>GFKDNSPISDTSFSLQLSQDGLQLTPASSSSESLSIIDVASDQNLFQTFIKEWRCKKRFSISLACEKIRSLTSSKTATIGSRFKQASSPQEIPIRDDGFPIKGCDDTLVVGLAVCWGGRDAYYFSLQKEQKHSEISASLVPPSLDPSLTLKDRMWYLQSCLRKESDKECSVVIYDFIQSYKILLLSCGISLEQSYEDPKVACWLLDPDSQEPTLHSIVTSFLPHELPLLEGMETSQGIQSLGLNAGSEHSGRYRASVESILIFNSMNQLNSLLQKENLQDVFRKVEMPSQYCLALLELNGIGFSTAECESQKHIMQAKLDAIETQAYQLAGHSFSFTSSDDIAEVLFLELKLPPNREMKNQGSKKTLGSTRRGIDNGRKLRLGRQFSTSKDVLNKLKALHPLPGLILEWRRITNAITKVVFPLQREKCLNPFLGMERIYPVSQSHTATGRITFTEPNIQNVPRDFEIKMPTLVGESPPSQAVGKGLLPMGRGKYKKGFSVNPRCQAQMEERAADRGMPFSISMRHAFVPFPGGSILAADYSQLELRILAHLSHDRRLIQVLNTGADVFRSIAAEWKMIEPESVGDDLRQQAKQICYGIIYGMGAKSLGEQMGIKENDAACYIDSFKSRYTGIN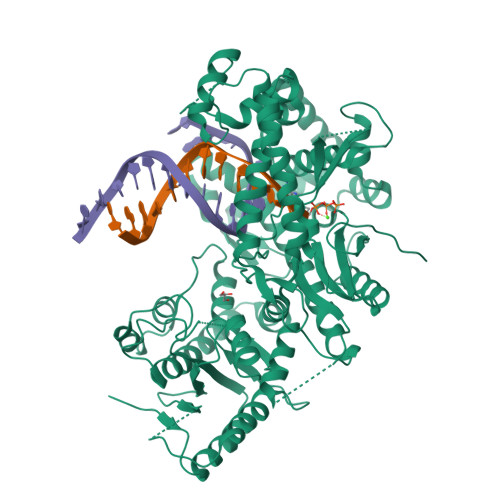QFMTETVKNCKRDGFVQTILGRRRYLPGIKDNNPYRKAHAERQAINTIVQGSAADIVKIATVNIQKQLETFHSTFKSHGHREGMLQSDQTGLSRKRKLQGMFCPIRGGFFILQLHDELLYEVAEEDVVQVAQIVKNEMESAVKLSVKLKVKVKIGASWGELKDFDV[4x]The second principal receptor for IgE, CD23, is a type II transmembrane glycoprotein with a C-type lectin-like domain (CTLD)4 (3, 4). In its membrane-bound form, CD23 consists of three CTLD “heads” connected to the membrane via a trimeric α-helical coiled-coil “stalk”. The interaction between CD23 and IgE is critical in the regulation of IgE synthesis, which can be up- or down-regulated depending on the oligomerization state of CD23 (2, 9, 10). We have determined the crystal structures of the human lectin-like head domain of CD23 in its Ca2+-free and Ca2+-bound forms, as well as the crystal structure of the Ca2+-bound head domain of CD23 in complex with a subfragment of IgE-Fc consisting of the dimer of Cϵ3 and Cϵ4 domains (Fcϵ3-4).

The Ca2+-free and Ca2+-soaked derCD23 crystals both belong to space group P1 and have four molecules within the asymmetric unit. Comparison of the Ca2+-free and Ca2+-bound derCD23 structures reveals that the only conformational differences are in loop 4 and, to a lesser degree, in loop 1. Although the four copies of loop 4 in the Ca2+-bound structure adopt similar conformations, two copies of this loop in the Ca2+-free structure adopt a different conformation, and the other two adopt yet another. These two different conformations of Ca2+-free derCD23 are not the result of different crystal packing interactions. In Ca2+-free “conformation 1,” two principal binding site residues (Glu-249 and Asp-270) are in a similar position to that observed in the Ca2+-bound structure, although the orientation of the Thr-251 side chain is different. In Ca2+-free “conformation 2,” only Glu-249 remains in a similar position when compared with the Ca2+-bound structure, although marked differences are seen for both Thr-251 and Asp-270. In the Ca2+-free structure, this distance is 6.1 Å in conformation 1 and 8.3 Å in conformation 2; Pro-250 is cis in the former and trans in the latter. The trans configuration of Pro-250 forms two hydrogen bonds with Arg-253, whereas cis Pro-250 cannot; consequently, both Arg-253 and Ser-254 are disordered when Pro-250 is cis (conformation 1), but are ordered, with Arg-253 pointing into a cavity between loops 1 and 4, when Pro-250 is trans (conformation 2). Thus, trans is apparently favored in the absence of Ca2+ or other factors.

>SGFVCNTCPEKWINFQRKCYYFGKGTKQWVHARYACDDMEGQLVSIHSPEEQDFLTKHASHTGSWIGLRNLDLKGEFIWVDGSHVDYSNWAPGEPTSRSQGEDCVMMRGSGRWNDAFCDRKLGAWVCDRLATCTPPASEGSAE[4x]> NVRFDLSSATSSSYKTFIKNLREALPKDGKVYDIPVLLST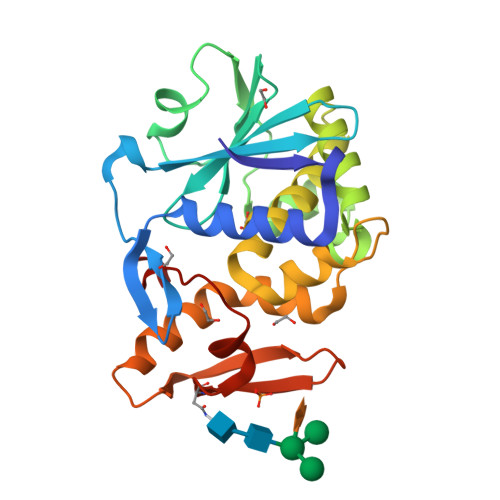VMDSRRFILIDLVNYDGQSITAAIDVLNVYIVAYSTGTVSYFFQQVPAQAPKLLFKGTQQRTLPYTGNYENLQTAAKKLRENIELGLPALDSAITTLFHYNAEAAASALLVLIQTTSEAARFRYIELQIANNVGTKFKPSQTIISLENNWSALSKQIQIAKNKNGQFETPVILIDPQGNRVQITNVTSNVVTQNIQLLLNIGATA>[2x]MFTGSIVAIVTPMDEKGNVCRASLKKLIDYHVASGTSAIVSVGTTGESATLN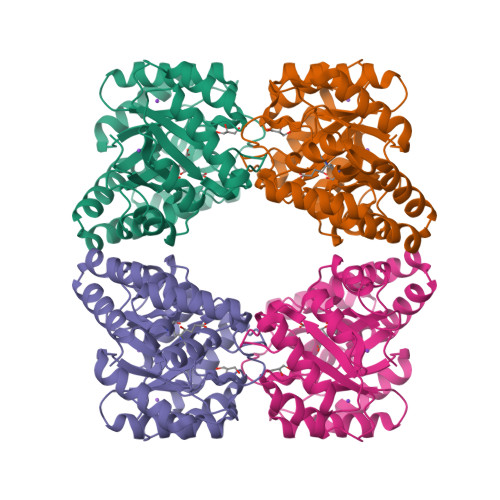HDEHADVVMMTLDLADGRIPVIAGTGANATAEAISLTQRFNDSGIVGCLTVTPYYNRPSQEGLYQHFKAIAEHTDLPQILYNVPSRTGCDLLPETVGRLAKVKNIIGIKEATGNLTRVNQIKELVSDDFVLLSGDDASALDFMQLGGHGVISVTANVAARDMAQMCKLAAEGHFAEARVINQRLMPLHNKLFVEPNPIPVKWACKELGLVATDTLRLPMTPITDSGRETVRAALKHAGLL>[6x]GALERLPDGPRIHVPRKTALRPTVARQVFQPAFAPAVLSKFDPRTDADVDEVAFSKHTSNQETLPPVFRMVAREYANRVFALLGRDNGRLSVKQALDGLEGMDPMDKNTSPGLPYTTLGMRRTDVVDWETATLIPFAAERLEKMNNKDFSDIVYQTFLKDELRPIEKVQAAKTRIVDVPPFEHCILGRQLLGKFASKFQTQPGLELGSAIGCDPDVHWTAFGVAMQGFERVYDVDYSNFDSTHSVAMFRLLAEEFFSEENGFDPLVKDYLESLAISKHAYEEKRYLITGGLPSGCAATSMLNTVMNNIIIRAGLYLTYKNFEFDDVKVLSYGDDLLVATNYQLNFDRVRTSLAKTGYKITPANKTSTFPLESTLEDVVFLKRKFKKEGPLYRPVMNREALEAMLSYYRPGTLSEKLTSITMLAVHSGKQEYDRLFAPFREVGVIVPTFESVEYRWRSLFW

The genome is replicated via a negative-sense RNA intermediate by 3Dpol, the viral RNA-dependent RNA polymerase (RdRP). For this, 3Dpol uses the viral protein 3B, in this context usually termed VPg (viral protein genome-linked), as a primer. Crystal structures have been reported of 3Dpol of the enteroviruses CVB3, PV, EV71, HRV1B, HRV14, and HRV16, and of the aphthovirus FMDV. These enzymes adopt a classical right hand architecture, with fingers, palm and thumb subdomains providing the correct geometrical arrangement of substrate molecules and metal ions at the polymerase active site for catalysis. Given its critical role in genome replication, 3Dpol is regarded as an attractive target for antiviral drugs.

Interestingly, the three virus pools each contained a single missense mutation compared to wild-type (wt) virus. These mutations were located either at nucleotide 7115 (A7115G) or 7127 (A7127G) resulting in amino acid changes M300V and I304V in the viral RdRP, 3Dpol, respectively. Markedly higher inhibition constants were observed for the two resistant mutants (M300V, 26.9 μM; I304V, 10.3 μM) as compared to that for the wt enzyme (1.3 μM). The apo structures of the EMCV M300V and I304V polymerase mutants were obtained using the same crystallization conditions as for the wt enzyme, yielding two different types of crystals for the mutants. The 3Dpol I304V mutant crystallized in the space group C2 with six polymerase molecules per a.u. and diffracted to 3.2 Å resolution. Structural comparisons showed that the mutant polymerases were almost identical to the wt enzyme. The main differences were concentrated in helix α10, which contains the mutated residues, and in the preceding loop B. The side chains of residues 300 and 304 participate in a large hydrophobic cluster linking α10 with helices α2 (Y75), α6 (F194, A195, F199), α7 (I210) and α8 (L241, F255 and F256), included in the inner fingers. The substitutions of the methionine and isoleucine side chains by the shorter valine in the mutants imply a weakening of these hydrophobic interactions. This could result in an increased flexibility of α10, including the disruption of the last helical turn, and of the B-loop, which appears to have a key role in GPC-N114 binding in EMCV 3Dpol. In contrast, I304 seems to be located relatively far away of the GPC-N114 binding cavity. The structures of the EMCV 3Dpol M300V and I304V mutants suggest that these mutations increase the flexibility of this loop, thereby affecting the binding site of GPC-N114 and probably losing a direct interaction with the shorter V300 side chain whilst retaining the ability to interact with the template-primer.> KRAALIQNLRDSYTETSSFAVIEEWAAGTLQEIEGIAKAAVEAHGTIRNSTYGRAQAEKSPEQLLGVLQRYQDLCHNVYCQAETIRTVIAIRIPEHKEADNLG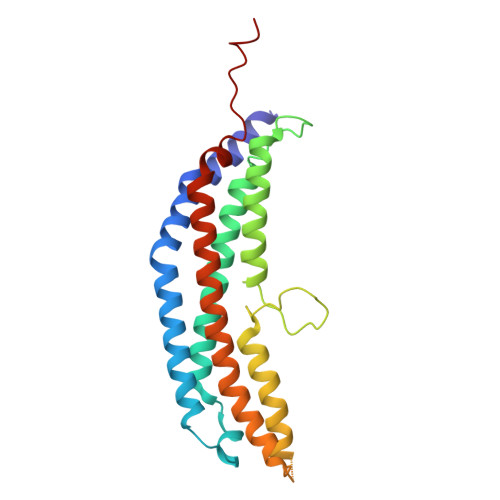VAVQHAVLKVIDELEIKTLGSGEKSGSGGAPTPIGMYALREYLSARSTVEDKLLGSVDAESGKTKGGSQSPSLLLELRQIDADFMLKVELATTHLSTMVRAVINAYLLNWKKLIQPRGGHLDVLYR>[6x]GKLSLQDVAELIRARACQRVVVMVGAGISTPSGIPDFRSPGSGLYSNLQQYDLPYPEAIFELPFFFHNPKPFF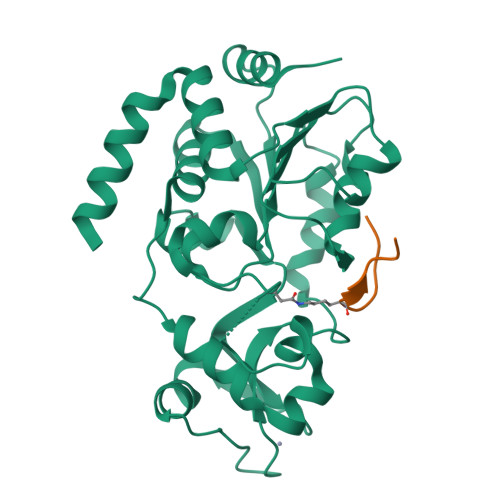TLAKELYPGNYKPNVTHYFLRLLHDKGLLLRLYTQNIDGLERVSGIPASKLVEAHGTFASATCTVCQRPFPGEDIRADVMADRVPRCPVCTGVVKPDIVFFGEPLPQRFLLHVVDFPMADLLLILGTSLEVEPFASLTEAVRSSVPRLLINRDLVGPLAWHPRSRDVAQLGDVVHGVESLVELLGWTEEMRDLVQRETGKL;>[6x]GKGGAXRHRKV>MFTMKLQSPEFQSLFTEGLKSLTELFVKENHELRIAGGAVRDLLNGVKPQDIDFATTATPTQMKEMFQSAGIRMINNRGEKHGTITARLHEENFEITTLRIDVTTDGRHAEVEFTTDWQKDAERRDLTINSMFLGFDGTLFDYFNGYEDLKNKKVRFVGHAKQRIQEDYLRILRYFRFYGRIVDKPGDHDPETLEAIAENAKGLAGISGERIWVELKKILVGNHVNHLIHLIYDLDVAPYIGLPANASLEEFDKVSKNVDGFSPKPVTLLASLFKVQDDVTKLDLRL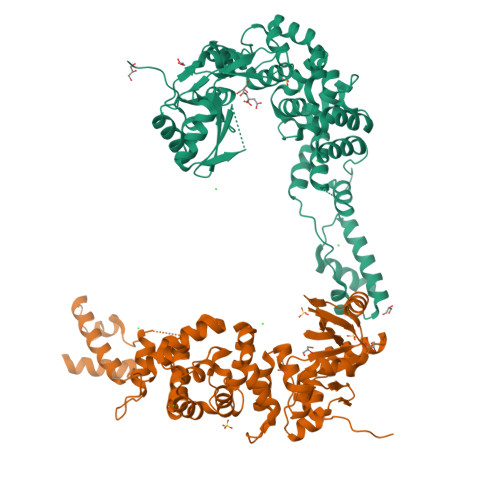KIAKEEKNLGLFIVKNRKDLIKATDSSDPLKPYQDFIIDSREPDATTRVCELLKYQGEHCLLKEMQQWSIPPFPVSGHDIRKVGISSGKEIGALLQQLREQWKKSGYQMEKDELLSYIKKTLEHHHHHH[2x]>MQIYEGKLTAE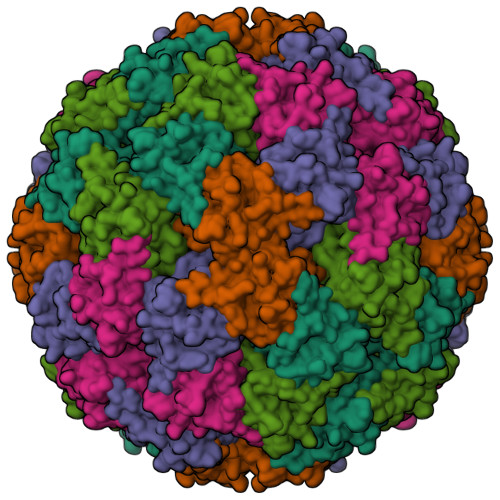GLRFGIVASRFNHALVDRLVEGAIDCIVRHGGREEDITLVRVPGSWEIPVAAGELARKEDIDAVIAIGVLIRGATPHFDYIASEVSKGLANLSLELRKPITFGVITADTLEQAIERAGTKHGNKGWEAALSAIEMANLFKSLR[5x]>MGSSHHHHHHSQDP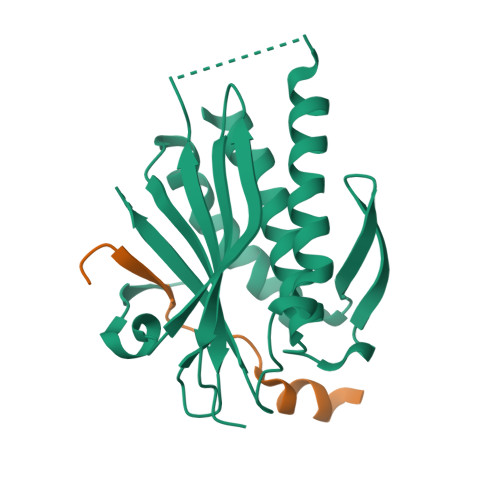NSMTTLTRQDLNFGQVVADVLCEFLEVAVHLILYVREVYPVGIFQKRKKYNVPVQMSCHPELNQYIQDTLHCVKPLLEKNDVEKVVVVILDKEHRPVEKFVFEITQPPLLSISSDSLLSHVEQLLAAFILKISVCDAVLDHNPPGCTFTVLVHTREAATRNMEKIQVIKDFPWILADEQDVHMHDPRLIPLKTMTSDILKMQLYVEERAHKGS[2x];>[2x]MLTPTPDSSPRSTSSPSQSKNGSFTPRTANILKPLMSPPSREEIMATLLDHD1-{3-[6-(1-methyl-1H-pyrazol-4-yl)-3,4-dihydroquinolin-1(2H)-yl]-1-[(3S)-oxolan-3-yl]-1,4,6,7-tetrahydro-5H-pyrazolo[4,3-c]pyridin-5-yl}ethan-1-one 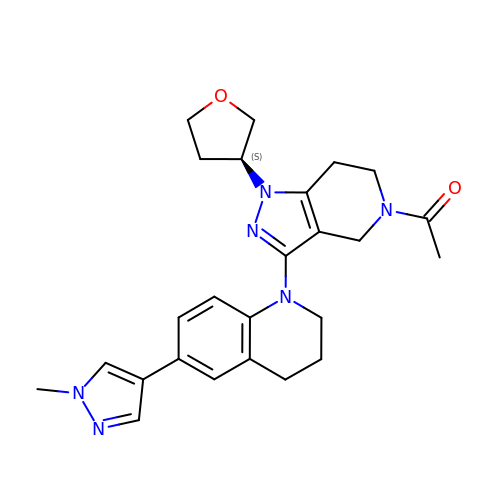| C25 H30 N6 O2 | OTJPVMSGEHNVNV-NRFANRHFSA-N Caudovirales, the taxonomic order for the tailed double-stranded DNA bacteriophages, is characterized by the presence of a tail—a host cell attachment organelle that is connected to the genome-containing spherical or elongated capsid via a neck. We describe cryo-EM structures of the neck, the neck-capsid and neck-tail junctions, and capsid of the Agrobacterium phage Milano. The tail to capsid junction involves a symmetry mismatch that is bridged by the neck, and is therefore crucial for the assembly of tailed phage. The extensive network of disulfide bonds within and between neck, collar, capsid and tail provides an exceptional structural stability to Milano.

The 15-fold, 12-fold and 3-fold symmetrized maps of the neck were used to build atomic models of the collar, portal, and neck devoid of capsid (portal + neck 1 + neck 2 + tail terminator + collar), respectively. Namely, the dodecameric portal ring (12 × gp7), which is embedded into the capsid shell, connects sequentially to the dodecameric neck 1 ring (12 × gp14), hexameric neck 2 ring (6 × gp15) and hexameric tail terminator ring (6 × gp18). The structures of portal, neck 2, and tail terminator rings of Milano show considerable similarity to their counterparts in other bacteriophages at both protomer and oligomeric levels. The β-sandwich domains form a positively charged “bowl”, which houses a negatively charged portal clip domain region31 thus strengthening the connection between the portal and the neck tube. The lumen of portal, neck 1, and neck 2 possesses a positive electrostatic potential resulting in a positive charge of the neck lumen —suitable to hold and position the end of the negatively charged linear dsDNA until the genome release.

>MLGIPLLTRKAALTPPAPSANPAKIFIRRFFSAGVAKNVVSYSNVMAAQRAMEHPVAFRCLDKLGLTVQSVKWDVGKDPQNTQVGDGGMSASQRKALQQILQRPNPTMSGAQLRYSAALSWACFGRMAFKVSVMSDGSVNAIWPLGIPFLKQKFDRYGDVESFQYGDEAGKETIPSFTKVEKNDKGRPIKNYAFMIVKPSINGAMNFDVQNTPLQAIGVPVALYDALMARAIDSADGTPNSKWLVTASRDLDDGQAKEVKEGIEETKPGGDNGGEIIFIAGTDVKVQEMKNDLSDIHSKVPLDDQARTIAGNFGIPIALLGFAGADGSKFANNYDESRKAFFEDTIEPGYLTPLEDGFSMFLCGAGYRVIFDRDSIPALRKSRADIAATYDKVTFITEEEKREVTGWPAKKEGQTQNDDA[12x]(Z)-N-[(1E)-1-carboxy-2-(2,3-dihydro-1H-indol-1-yl)ethylidene]{3-hydroxy-2-methyl-5-[(phosphonooxy)methyl]pyridin-4(1H)-ylidene}methanaminium 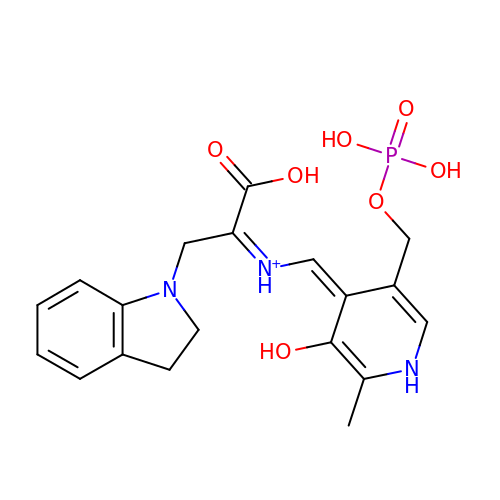| C19 H23 N3 O7 P | MAJPVKFOYDGVKD-LNHPUNTFSA-O>SSFHATTIFAVQHKGRSAMSGDGQVTFGQAVVMKHTARKVRKLFNGKVLAGFAGSVADAFTLFEKFEAKLEEYNGNLKRAAVELAKEWRSDKVLRKLEAMLIVMNQDTLLLVSGTGEVIEPDDGILAIGSGGNYALAAGRAL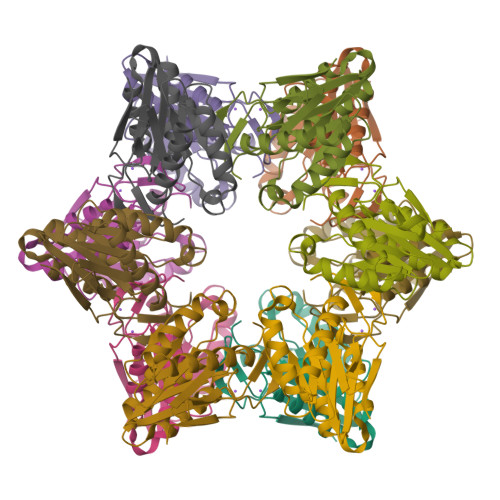KKHAGESMSASEIARAALETAGEICVYTNDQIILEELE[12x]4-(2-hydroxyethylcarbamoyl)benzoic acid | C10 H11 N 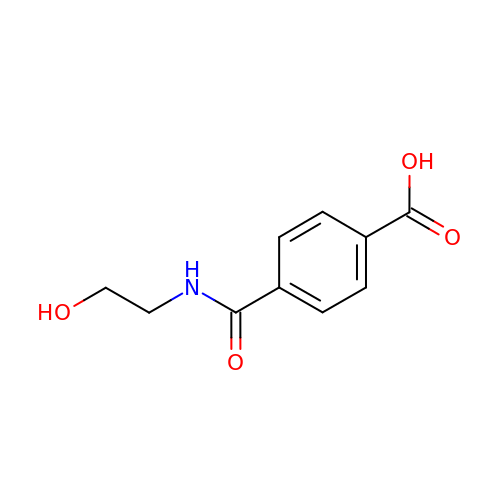O4 | HGTVOBHNUAVYMK-UHFFFAOYSA-N>MQKAVVMDEQAIRRALTRIAHEIIERNKGIDGCVLVGIKTRGIYLARRLAERIEQIEGASVPVGELDITLYRDDLTVKTDDHEPLVKGTNVPFPVTERNVILVDDVLFTGRTVRAAMDAVMDLGRPARIQLAVLVDRGHRELPIRADFVGKNVPTSRSE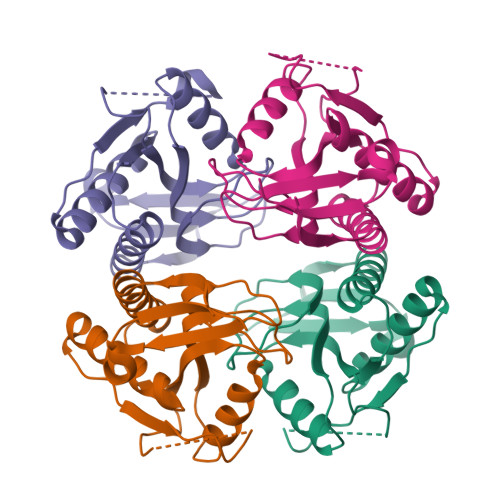LIVVELSEVDGIDQVSIHEK[4x]> MEWAAKKTNSLTSSSERTWKANLLVPVEDPRELMGTFDFLRDITYPKGSVKLLGLAGNTDKENLLSQLPSISEGFQEEGVFSSWTIIDTAEFEENLVVGMEALTGSFFRPSILFLRLPENRDRDEEIREIIRKASMYRMGVLLFSKHPQAGLGRQNLINLWIENRGLDWDISMELGNMDLALLIAYKLKSNW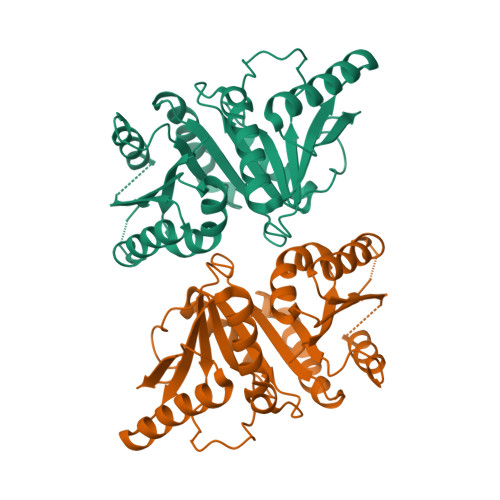KASLSFMTFAPTAIQAQAAENFLQSLAELARIPNVKMQVLRENPIKSSKLPFASLHIFSLDPNPDLDLARHLMEKAGSSCIFALDSGEENALALLEHHHHHH>GDAVTILSATECWDLLKSVALGRIVTTVDNTSHIFPINFVVQNRTVLFRTAEGTKLVSAAINNNVLFEADDHDVEQGW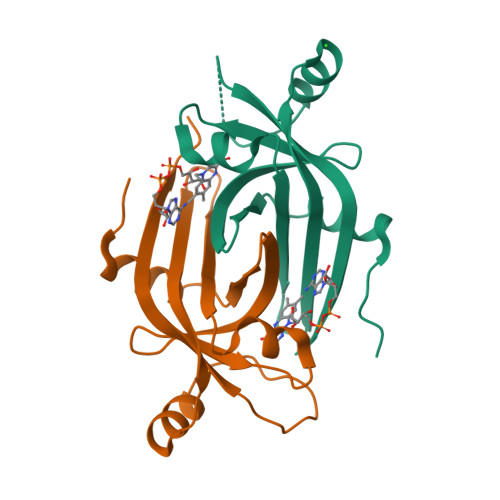SVIVRGVARTVRDEADLAEAQRAELLPWTATAKTHWVRVLPTQITGRRFRFGPE[20x]> MSSIDNDSDVDLTEDLAVAKIVKENPVARKMVRYILSRGESQNSIITRNKLQSVIHEAAREENIAKPSFSKMFMDINAIL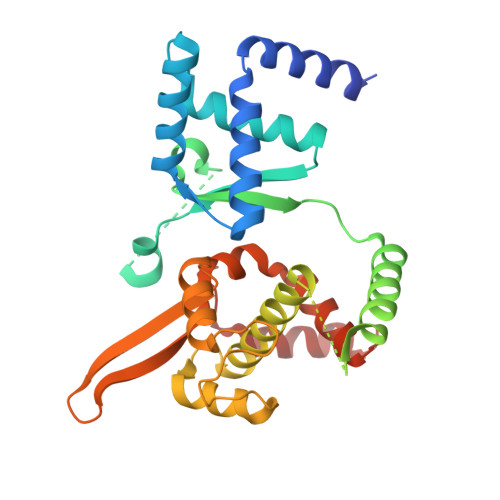YNVYGFELQGLPSKNNMNAGGNGSNSNTNKSMPEPLGHRAQKFILLNNVPHSKNFDDFKILQSAHTYEELIVTGEYIGDDIASGTSNTLESKLSTDRDLVYKGVLSVILCIVFFSKNNILHQELIKFLETFGIPSDGSKIAILNITIEDLIKSLEKREYIVRLEEKSDTDGEVISYRIGRRTQAELGLESLEKLVQEIMGLEKEQTKSLHDDIIKSIGDSYSI> MELKHSISDYTEAEFLQLVTTICNADTSSEEELVKLVTHFEEMTEHPSGSDLIYYPKEGDDDSPSGIVNTVKQWRAANGKSGFKQG;> MESKRNKPGKATGKGKPVGDKWLDDAGKDSGAPIPDRIADKLRDKEFKSFDDFRKAVWEEVSKDPELSKNLNPSNKSSVSKGYSPATP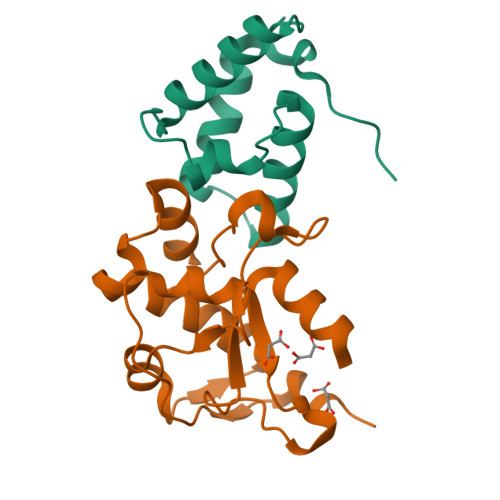KNQQVGGRKVYELHHDKPISQGGEVYDMDNIRVTTPKRHIDIHRGK>SNATFTCDELKGLEHPYEVLGNGDALAENREELNKLTNDAALVLASRLVLECPVNELKDFAHAIEAARMPQDDSDTFHSFLFQAYQVKKRIISLLDPRNINPHSMILEKEFDGELFNNFNKLAIDVLTNNEVAIALRLAETTPAQDRSRVSQNINNIFPQSLFAAKVGHAFAVRRDIERLLLGDRPDQFFSSREFKIDSCIEFASLFNVINDKESSIAGKLALRTPAENRTDVVMKIKGFCAEDSELAIKVQSAFALRRDIERNLLGDNPEQFFSSRDFSVDLCLEFAILFPELLKGHEQAIGEKLAKLDAKVRSDISRKLEMINGAAH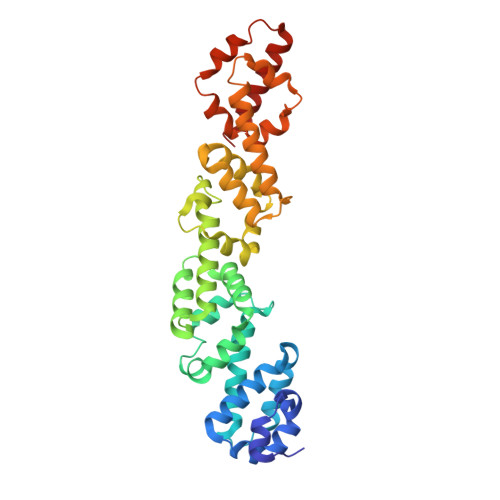EQ[2x]> MTATVLLEVPFSARGDRIPDAVAELRTREPIRKVRTITGAEAWLVSSYALCTQVLEDRRFSMKETAAAGAPRLNALTVPPEVVNNMGNIADAGLRKAVMKAITPKAPGLEQFLRDTANSLLDNLITEGAPADLRNDFADPLATALHCKVLGIPQEDGPKLFRSLSIAFMSSADPIPAAKINWDRDIEYMAGILENPNITTGLMGELSRLRKDPAYSHVSDELFATIGVTFFGGGVISTGSFLTTALISLIQRPQLRNLLHEKPELIPAGVEELLRINLSFADGLPRLATADIQVGDVLVRKGELVLVLLEGANFDPEHFPNPGSIELDRPNPTSHLAFGRGQHFCPGSALGRRHAQIGIEALLKKMPGVDLAVPIDQLVWRTRFQRRIPERLP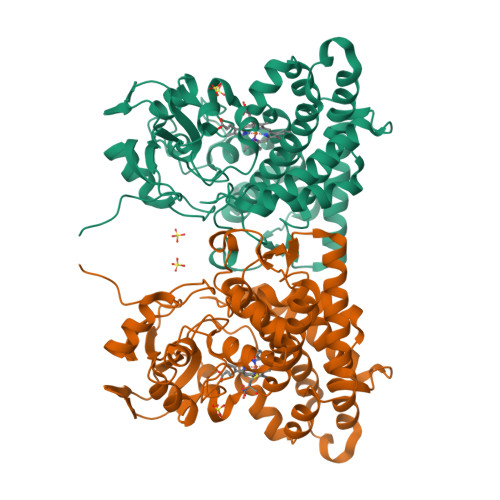VLW>HHHHHHAVAKDSTESKSWEPFSLSPIKDPQALHAALCSKNVIPVTSTLEDLLPATQAQHVFIKRGTFHSYNWTIKGRSLNMDRLRETCQSLVDRHSILRTSFVEHEGHPIQLVLANLDVKVREVQCWPGEDPMEVCKALWDGKDWPTLNVLGGSLPVRFTLVSCPGNEHVVLTIQISHSQWDGVSIPKLFSDFAAIYNQTPLPPTSDFAHYLYHRVSSAREDVQQDPTFQFWRHYLDGAKMAVPFAPRALTLCAEPAAAAQSGQTLWTFKGIVPPTLPSGITMATLVKAATALFLSYHLGSRDVVFGHTVNGRNLPMDNIESLLGCTLNFVPLRVTFPEDSTDWTVMDLLHHTQTQYTRALSHEHVELRDIFQHS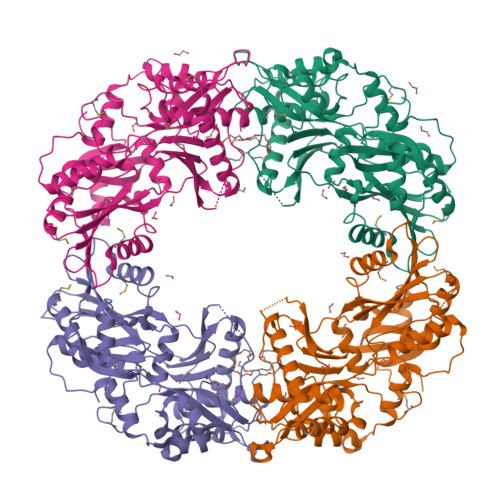TNWPAETPLSLIVQHQNIDLSFSLPLRGSSVSGDGEDDSSLDVQYSKFARFDPLDEVWIFTEPHADRLEVQVCANSRVLGQEQATELANNISAIITKFSTDPTARLLDITF[4x]> MRVGLVGWRGMVGSVLMQRMVEERDFDLIEPVFFSTSQIGVPAPNFGKDAGMLHDAFDIESLKQLDAVITCQGGSYTEKVYPALRQAGWKGYWIDAASTLRMDKEAIITLDPVNLKQILHGIHHGTKTFVGGNCTVSLMLMALGGLYERGLVEWMSAMTYQAASGAGAQNMRELISQMGVINDAVSSELANPASSILDIDKKVAETMR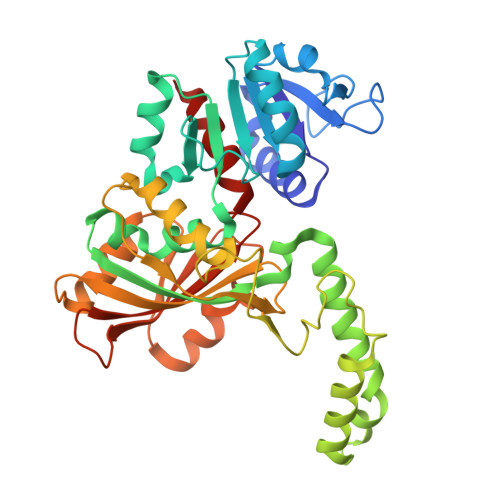SGSFPTDNFGVPLAGSLIPWIDVKRDNGQSKEEWKAGVEANKILGLQDSPVPIDGTCVRIGAMRCHSQALTIKLKQNIPLDEIEEMIATHNDWVKVIPNERDITARELTPAKVTGTLSVPVGRLRKMAMGDDFLNAFTVGDQLLWGAAEPLRRTLRIILAEK N-phenylnaphthalen-1-amine | C16 H13 N | 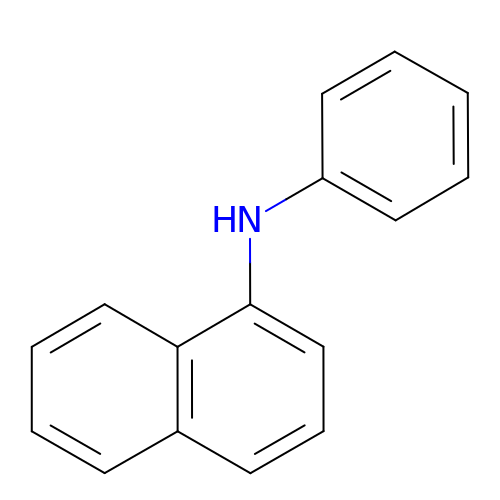XQVWYOYUZDUNRW-UHFFFAOYSA-N>GSFIDIEFPEWFHEGLSRHQAENLLMGKDIGFFIIRASQSSPGDFSISVRHEDDVQHFKVMRDTKGNYFLWTEKFPSLNKLVDYYRTTSISKQKQVFLRD[4x];>[4x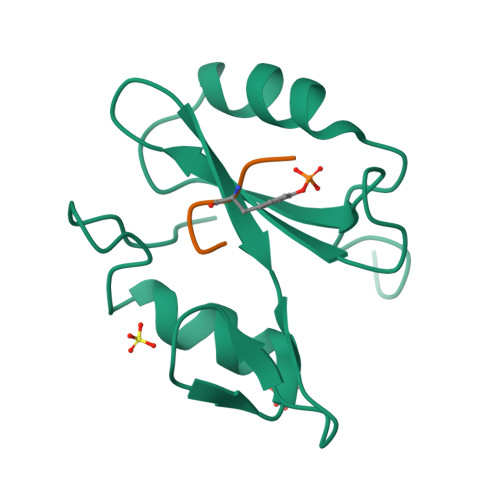]XDDYVNV>[2x]QCPAIHVFGARETTVSQGYGSSATVVNLVIQAHP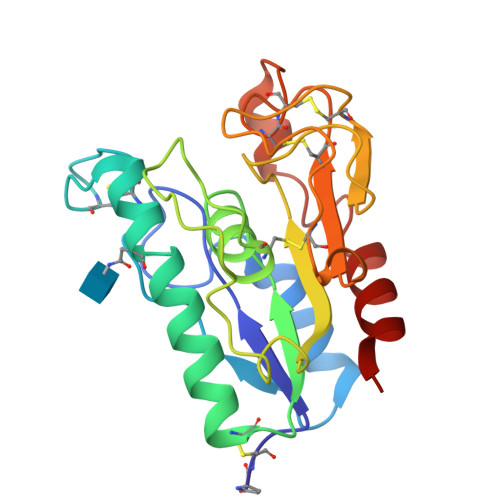GTTSEAIVYPACGGQASCGGISYANSVVNGTNAAAAAINNFHNSCPDTQLVLVGYSQGAQIFDNALCGGGDPGEGITNTAVPLTAGAVSAVKAAIFMGDPRNIHGLPYNVGTCTTQGFDARPAGFVCPSASKIKSYCDAADPYCCTGNDPNVHQGYGQEYGQQALAFINSQLS> SLT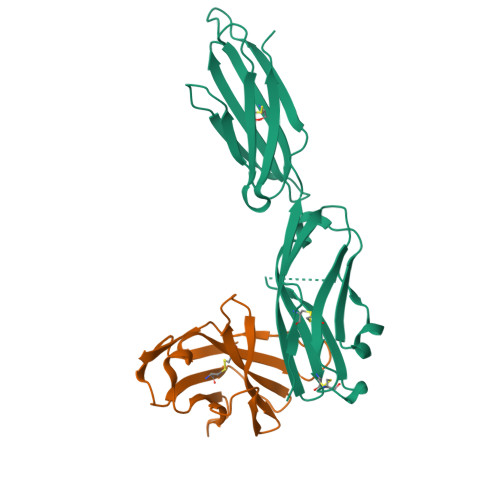FYPAWLTVSEGANATFTCSLSNWSEDLMLNWNRLSPSNQTEKQAAFSNGLSQPVQDARFQIIQLPNRHDFHMNILDTRRNDSGIYLCGAISRHPKAKIEESPGAELVVTERILE;> LFTVTAPKEVYTVDVGSSVSLECDFDRRECTELEGIRASLQKVENDTSLQSERATLLEEQLPLGKALFHIPSVQVRDSGQYRCLVICGAAWDYKYLTVKVKASYMRIDTRILEVPGTGEVQLTCQARGYPLAEVSWQNVSVPANTSHIRTPEGLYQVTSVLRLKPQPSRNFSCMFWNAHMKELTSAIIDPLSRMEPKVPRT SNARE (soluble N-ethylmaleimide-sensitive factor (NSF) attachment protein receptor) proteins drive membrane fusion at different cell compartments as their core domains zipper into a parallel four-helix bundle. After fusion, these bundles are disassembled by the AAA+ (ATPase associated with diverse cellular activities) protein Sec18/NSF and its adaptor Sec17/α-SNAP to make them available for subsequent rounds of membrane fusion. The disassembly requires multiple ATP hydrolysis events in the presence of Mg2+; as few as six ATP hydrolysis events are sufficient. The side-loading and side-release mechanism explains how Sec18/NSF can disassemble SNAREs with constrained topologies.

To address this topological challenge, we next determined structures of the y20S complex after initiating Sec18 hydrolysis by adding Mg2+ (referred to as the ‘hydrolyzing condition’). Informed by a fluorescent protein disassembly assay, we initiated the disassembly reaction and waited 7 s before sample vitrification. The D1 ring is also flat in all these substrate-free classes, with all D1 protomers bound to ADP. In the D2 ring, all protomers are still ATP bound, consistent with their role in oligomerization. Class 2 has a well-resolved hexameric configuration with a coordinated split in class 2 in the D1 and D2 rings. This split spans ~20 Å between protomers and is large enough to accommodate a polypeptide chain entering or leaving the rings. The coordinated split in the D1 and D2 domain rings allows the processed SNARE substrate to be released from the side. This side-release mechanism, thus, addresses one part of the topological challenge stated above; threading occurs but the substrate exits from the side, avoiding the membrane domains and linkages in SNARE proteins.

>[6x]GAHMFKIPGFGKAAANHTPPDMTNMDTRTRHLKVSNCPNNSYALANVAAVSPNDFPNNIYIIIDNLFVFTTRHSNDIPPGTIGFNGNQRTWGGWSLNQDVQAKAFDLFKYSGKQSYLGSIDIDISFRARGKAVSTVFDQDELAKQFVRCYESQIFSPTQYLIMEFQGHFFDLKIRNVQAIDLGDIEPTSAVATGIETKGILTKQTQINFFKGRDGLVNLKSSNSLRPRSNAVIRPDFKFEDLGVGGLDKEFTKIFRRAFASRIFPPSVIEKLGISHVKGLLLYGPPGTGKTLIARKIGTMLNAKEPKIVNGPEILSKYVGSSEENIRNLFKDAEAEYRAKGEESSLHIIIFDELDSVFKQRGSRGDGTGVGDNVVNQLLAKMDGVDQLNNILVIGMTNRKDLIDSALLRPGRFEVQVEIHLPDEKGRLQIFDIQTKKMRENNMMSDDVNLAELAALTKNFSGAEIEGLVKSASSFAINKTVNIGKGATKLNTKDIAKLKVTREDFLNALNDVTPAFGISEEDLKTCVEGGMMLYSERVNSILKNGARYVRQVRESDKSRLVSLLIHGPAGSGKTALAAEIALKSGFPFIRLISPNELSGMSESAKIAYIDNTFRDAYKSPLNILVIDSLETLVDWVPIGPRFSNNILQMLKVALKRKPPQDRRLLIMTTTSAYSVLQQMDILSCFDNEIAVPNMTNLDELNNVMIESNFLDDAGRVKVINELSRSCPNFNVGIKKTLTNIETARHDEDPVNELVELMTQSA>[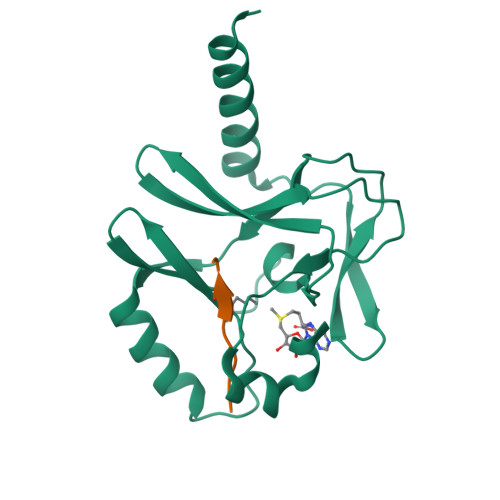2x]KSKAELQSEERKRIDELIESGKEEGMKIDLIDGKGRGVIATKQFSRGDFVVEYHGDLIEITDAKKREALYAQDPSTGCYMYYFQYLSKTYCVDATRETNRLGRLINHSKSGNCQTKLHDIDGVPHLILIASRDIAAGEELLYDYGDRSKASIEAHPWLKH;>[2x]KRHRLVLR3-HYDROXY-TETRADECANOIC ACID | C14 H28 O3 | 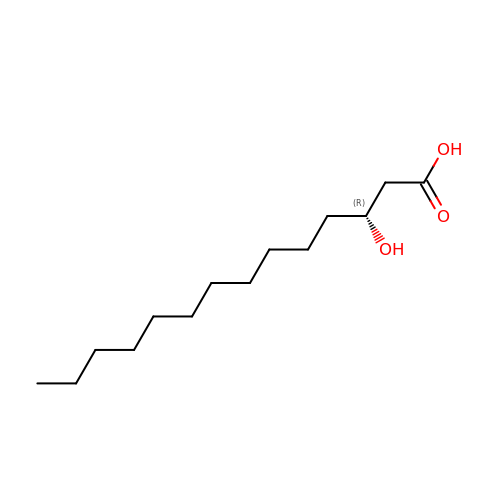ATRNZOYKSNPPBF-CYBMUJFWSA-N>GAMEPLRVLELYSGVGG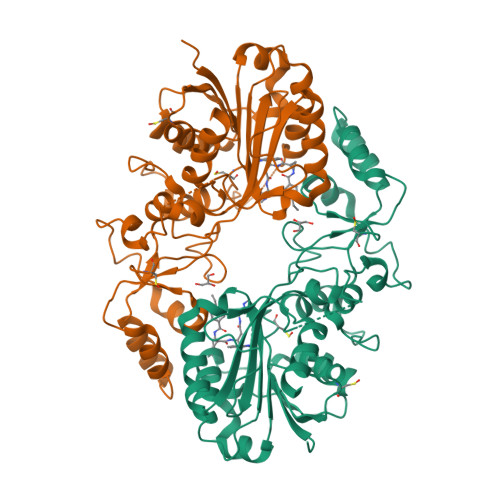MHHALRESCIPAQVVAAIDVNTVANEVYKYNFPHTQLLAKTIEGITLEEFDRLSFDMILMSPPCQPFTRIGRQGDMTDSRTNSFLHILDILPRLQKLPKYILLENVKGFEVSSTRDLLIQTIENCGFQYQEFLLSPTSLGIPNSRLRYFLIAKLQSEPLPFQAPGQVLMEFPKIESEIHRKNQQDSDLSVKMLKDFLEDDTDVNQYLLPPKSLLRYALLLDIVQPTCRRSVCFTKGYGSYIEGTGSVLQTAEDVQVENIYKSLTNLSQEEQITKLLILKLRYFTPKEIANLLGFPPEFGFPEKITVKQRYRLLGNSLNVHVVAKLIKILYE[2x]4-[[GLUTAMIC ACID]-CARBONYL]-BENZENE-SULFONYL-D-PROLINE | C17 H20 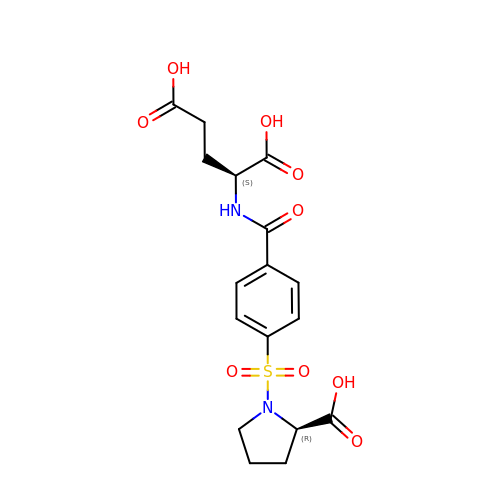N2 O9 S | NDDOUBGQRWFVQM-QWHCGFSZSA-N>MDINASRALANVYDLPDDFFPKIDDLVRDAKDALEPYWKSDSIKKHVLIATHFVDLIEDFWQTTQGMHEIAESLRAVGGSGGAEIHAHLKAYAKINEESLDRARRLLWWHYNCLLWGEAQVTNYISRLRTWLSTPEKYRGRDAPTIEAITRPIQVAQGGRKTTTGTRKPRGLEPRRRKVKTTVVYGRRRSKSRERRAPTPQRAGSP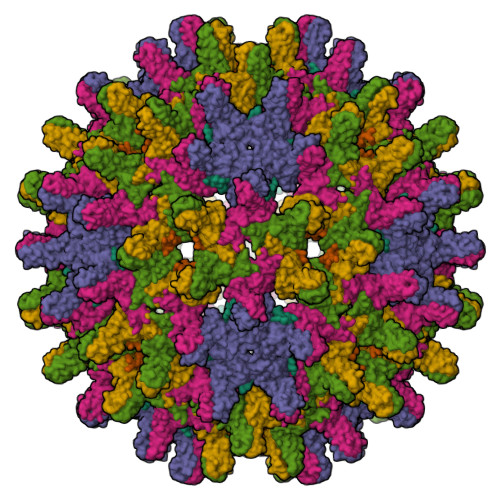LPRSSSSHHRSPSPRK[6x]>MKHHHHHPMVPSYDSFDSEDYPAALPNHKPKGTFKDYVRDRADLNKDKPVIPAAALAGYTGSGPIQLWQFLLELLTDKSSQSFISWTGDGWEFKLSDPDEVARRWGKRKNKPKMNYEKLSRGLRYYY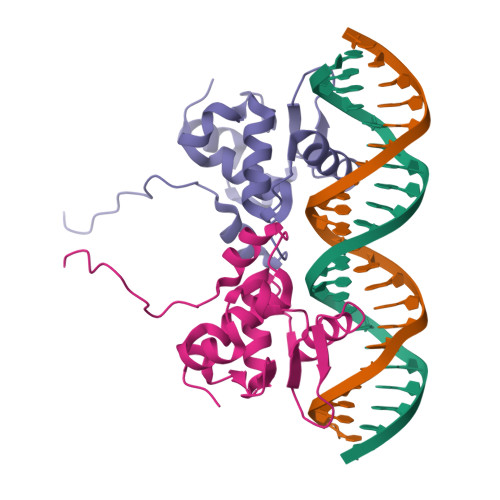DKNIIHKTAGKRYVYRFVSDLQSLLGYTPEELHAMLDVKPDADE[2x]>[2x]MHHHHHHGENLYFQGSAPYASLTEIEHLVQSVCKSYRETCQLRLEDLLRQRSNIFSREEVTGYQRKSMWEMWERCAHHLTE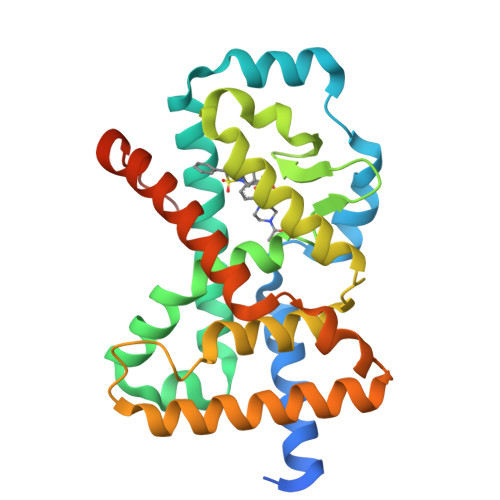AIQYVVEFAKRLSGFMELCQNDQIVLLKAGAMEVVLVRMCRAYNADNRTVFFEGKYGGMELFRALGCSELISSIFDFSHSLSALHFSEDEIALYTALVLINAHRPGLQEKRKVEQLQYNLELAFHHHLCKTHRQSILAKLPPKGKLRSLCSQHVERLQIFQHLHPIVVQAAFPPLYKELFSGNS;> VERLQIFQHLHPI>MSLQGIHLSDLSYKHAILKESQYTIKRDVGTTTAVTPSSLQQEITLLCGEILYAKHADYKYAAEIGIQYISTALGSERVQQILRNSGSEVQVVLTRTYSLGKIKNNKGEDLQMLDIHGVEK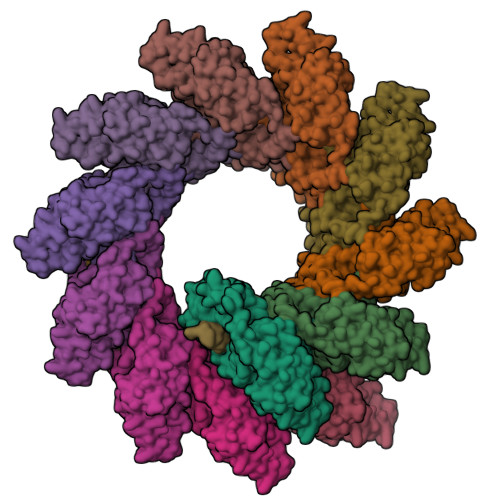SWVEEIDKEARKTMATLLKESSGNIPQNQRPSAPDTPIILLCVGALIFTKLASTIEVGLETTVRRANRVLSDALKRYPRMDIPKIARSFYDLFEQKVYHRSLFIEYGKALGSSSTGSKAESLFVNIFMQAYGAGQTMLRWGVIARSSNNIMLGHVSVQAELKQVTEVYDLVREMGPESGLLHLRQSPKAGLLSLANCPNFASVVLGNASGLGIIGMYRGRVPNTELFSAAESYAKSLKESNKINFSSLGLTDEEKEAAEHFLNVSDDSQNDYEKHHHHHH[12x]> MQAGPALMSEVA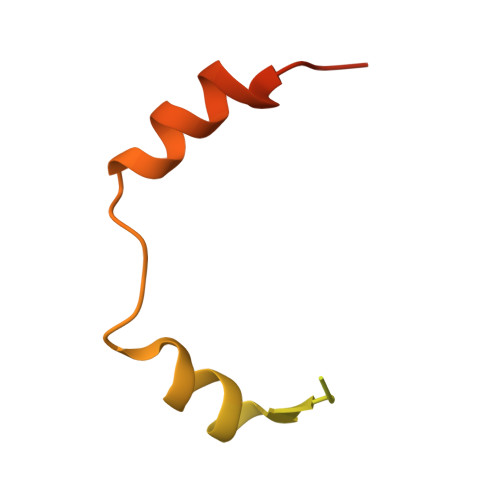SRELRNDTAGVLRRVRAGEDVTITVSGRPVAVLTPVRPRRRRWLSKTEFLSRLRGAQADPGLRNDLAVLAGDTTEDLGPIR2N-methyl-4N-(4-oxidanylcyclohexyl)-5-[(1S)-1-phenylethyl]furan-2,4-dicarboxamide 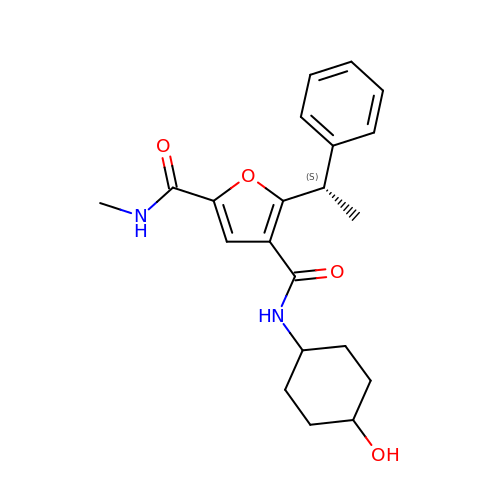| C21 H26 N2 O4 | BRAMSTZRKUJRKS-BPUTZDHNSA-N>[2x]HMLEGGSGGSGGSTIYH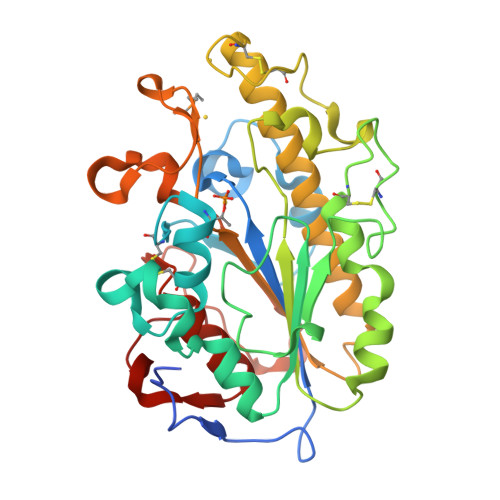AKDAVQATKPDMRKPRLVVFVVGETARADHVSFNGYERDTFPQLAKIDGVTNFSNVTSCGTSTAYSVPCMFSYLGADEYDVDTAKYQENVLDTLDRLGVSILWRDNNSDSKGVMDKLPKAQFADYKSATNNAICNTNPYNECRDVGMLVGLDDFVAANNGKDMLIMLHQMGNHGPAYFKRYDEKFAKFTPVCEGNELAKCEHQSLINAYDNALLATDDFIAQSIQWLQTHSNAYDVSMLYVSDHGESLGENGVYLHGMPNAFAPKEQRSVPAFFWTDKQTGITPMATDTVLTHDAITPTLLKLFDVTADKVKDRTAFIR>[16x]GSPGISGGGGGSASPNSPKDNTWIQAASLTWLMDMSSLLYQLISTRIPSFASPNGLHMREQTIDSNTGQIQIDNEHRLLRWDRRPPNDIFLNGFIPRVTNQNLSPVEDTHLLNYLRTNSPSIFVSTTRARYNNLGLEITPWTPHSANNNIIYRYEIFAPGGIDINASFSRNHNPFPNQDEITFPGGIRP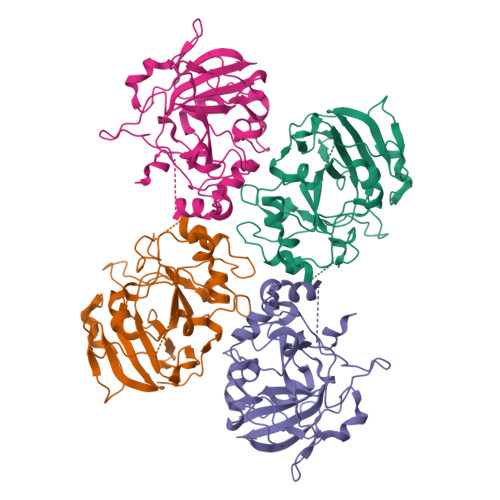EFIRSTYEYHNGEIVRIWINPNFINPSTLNDVSGPSNISKVFWHENHSEGNNMDSKGFILDLDYNQDFDMFAPNGEIPNNNLLNNNSLNVIQNSEYQIKNKK>SESSIVNACLRYLGYSKSMCHEKMPIFMDIAFIEYCFNLSLDPSSFQGGASQQILWEYSLISNALERLENIELERQNCMREDGLSKYTNSLLLNKETLNNEALKLYSCAKAGICRWMAFHFLEQEPIDHINFTKFLQDWGSHNEKEMEALQRLSKHKIRKRLIYVSQHKKKMPWSKFNSVLSRYIQCTKLQLEVFCDYDFKQREI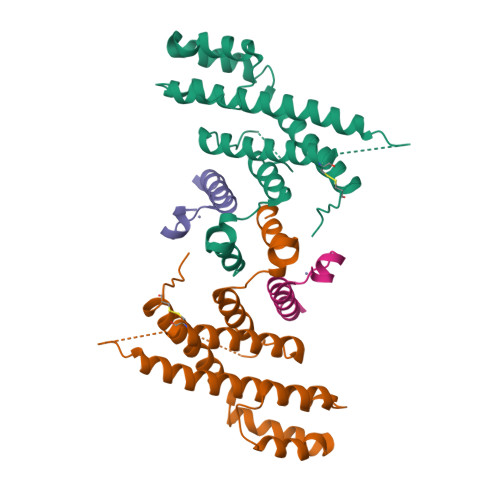VKMLTSNIN[2x];>SEACEMCRLGLPHGSFFELLRDWKKIEEFRNKS[2x]>MNNVEKAIEALKKGEIILVYDSDEREGETDMVVASQFITPEHIRIMRKDAGGLICTALHPDICNKLGIPFMVDILEFASQKFKV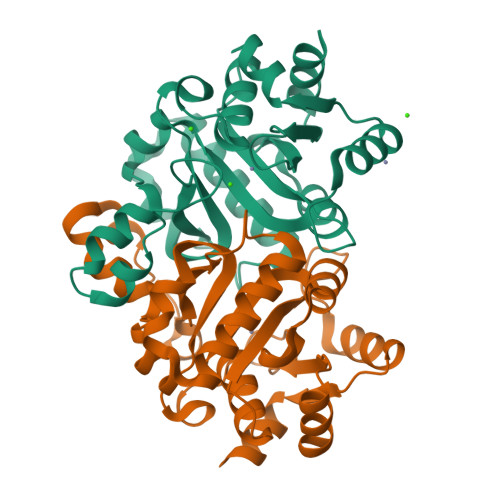LRELYPNDIPYDEKSSFSITINHRKTFTGITDNDRAFTIKKLAELVKEGRFNDFGKEFRSPGSVTLLRAAEGLVKNRQGHTEMTVALAELANLVPITTICEMMGDDGNAMSKNETKRYAEKHNLIYLSGEEIINYYLDKYLKD[2x]> AEMPKRKFTIDDFDIVRPLGKGKFGNVYLAREKQNKFIMALKVLFKSQLEKEGVEHQLRREIEIQSHLRHPNILRMYN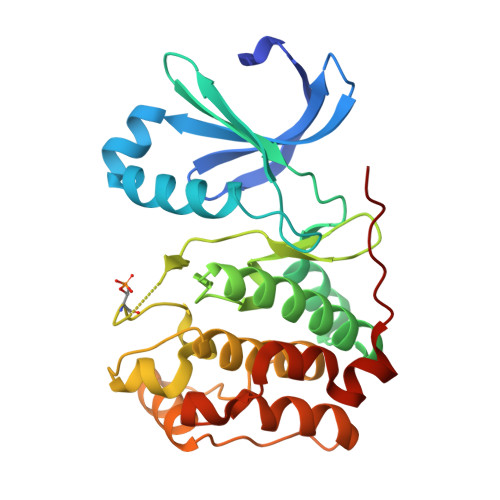YFHDRKRIYLMLEFAPRGELYKELQKHGRFDEQRSATFMEELADALHYCHERKVIHRDIKPENLLMGYKGELKIADFGWSVHAPSLRRRTMCGTLDYLPPEMIEGKTHDEKVDLWCAGVLCYEFLVGMPPFDSPSHTETHRRIVNVDLKFPPFLSDGSKDLISKLLRYHPPQRLPLKGVMEHPWVKANSRRVLPPVYQ>MASNQEEVKVYGMMASPFVSRVEIALKLKGVEYKYELEKFGNFSDTLIKYNPVYKKVPVFVHNDRPISESLVILEYIDETWKQNPLLPSDPYKRALVRFWTKFIDDKCLSAARKATFSIDEKEREKGIEETEEAFQILENELKDKFFGGDEIGIVDIAGIFIAFWFPIVQEATRLKLFTSEKFPKLHKWSEDLSNHPIVKEILPPRESLLAYFKARYESLTASK[2x]

GSTs are multifunctional enzymes that have evolved from a thioredoxin-like ancestor gene. GSTs catalyze the nucleophilic attack of reduced GSH (γ-Glu–Cys–Gly) on the electrophilic center of these compounds, leading to the formation of GSH conjugates that display higher solubility and reduced toxicity. Each subunit displays two ligand-binding sites: a G-site and an H-site. In the present work, DNA shuffling was employed for the design and creation of a library of tau class GSTs (GSTUs) from abiotic stress-treated Phaseolus vulgaris and Glycine max.

The enzyme that resulted from DNA shuffling, which was denoted as PvGmGSTUG in accordance with the nomenclature proposed by Edwards et al. (2000), clustered together with the tau class GSTs. PvGmGSTUG was crystallized with two molecules in the crystallographic asymmetric unit that followed the typical dimer formation found in other GSTs. Residues 1–5 in both chains, and the fragments 214–224 (chain B), and 216–224 (chain A) were not included in the structure owing to high disorder. The analysis revealed that each monomer of PvGmGSTUG consists of two distinct domains: at the N-terminal region a small α/β thioredoxin-like domain with βαβαββα folding topology is formed. At the C-terminal region a large helical domain is formed. In PvGmGSTUG, a Phe residue replaces Lys, a change that could affect the orientation of GSH. In PvGmGSTUG, it is replaced by a Cys residue, a change that could make the H-site more open and possibly alter its binding properties. A fourth hydrophobic residue, Leu134, is replaced by Ala134 in PvGmGSTUG, a change that may contribute to weakening of the interface. Structural examination revealed that the key residue bridging the dimer interface, Asp105, may play an important role in inter-subunit communication. This residue could interact with Lys102 from the second subunit, forming a strong salt bridge.>MKKLFLVFWWHMHQPLYREPYTGEYLLPWTFFHAVKDYYDMPAYLKDFEIKLNFNLTPVLIDQIQEYAQGKAKDVFLEAIRKDPDDLEKEEVEKLIEFTKLNYEKPIYRFERIRELMNKEKLNREELLDLQTLNLLAWCGRTLRKDLKDLLNKGRNYTQEEKEYVLNKYFEIIKKTLSIYREIKEEGKGSVSTSPYYHPLIPILLNPNCVYETTPNVKIPDFAVSFREDASKHVELAKEKYFEIFGEHPVYMWPPEASV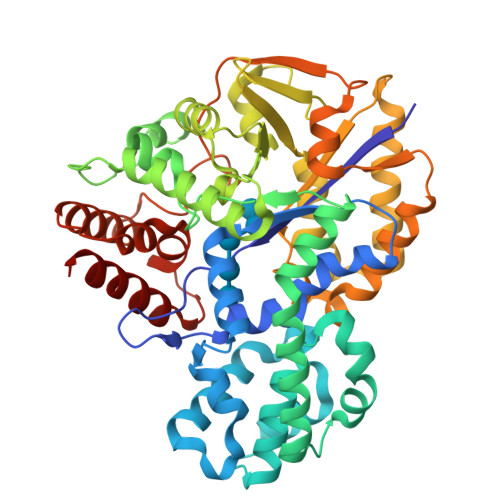SNEALELYYEKGINMLATDEVILKNSVERASPYLRYYFRELISVFFRDKTLSDLIGFSYHAWNAEDAVRDFIGRLKKIHESVDFQPVVFVVLNGENCWEYYEENGIPFLEKLYSTLEKEEWIETLTLEEAMRKEDVKTEVIESVKAGTWFDGNFLKWIGNKEKNEYWKILIEAKKKAKNDYILVAEGSDWFWWQGEEKAPFVEVFDKLFRSFVRRAQE[2x]>[4x]MSPEKQPLPAALVGSHVRAAAGTPADLATDRKFWTGLSRAVQERIADDWERTREAYGAARQQHYFSAEFLMGRALLNNLTNLGLVDEAAAATRELGHELTDILEIENDAALGNGGLGRLAACFLDSAVTQDYPVTGYGLLYRFGLFRQSFNEGFQVEKPDPWREEEYPFTIRRASDQLVVCFDDMKTRAIPYDMPITGYGTHNVGTLRLWKAEPWEEFDYDAFNAQRFTDAIIERERVSDICRVLYPNDTTYEGKKLRVRQQYFFTSASLQAMIQDHLAHH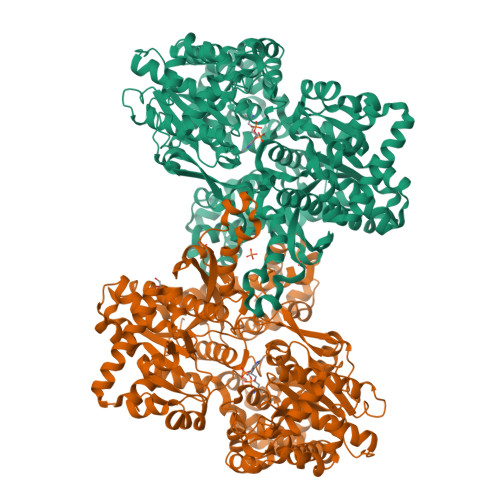KDLSNFAEFHSVQLNDTHPVLAIPELMRLLMDEHDMGWEESWAIVSKTFAYTNHTVLTEALEQWDEQIFQQLFWRVWEIIAEIDRRFRLERAADGLDEETINRMAPIQHGTVHMAWIACYAAYSINGVAALHTEIIKAETLADWYALWPEKFNNKTNGVTPRRWLRMINPGLSDLLTRLSGSDDWVTDLDELKKLRSYADDKSVLEELRAIKAANKQDFAEWILERQGIEIDPESIFDVQIKRLHEYKRQLMNALYVLDLYFRIKEDGLTDIPARTVIFGAKAAPGYVRAKAIIKLINSIADLVNNDPEVSPLLKVVFVENYNVSPAEHILPASDVSEQISTAGKEASGTSNMKFMMNGALTLGTMDGANVEIVDSVGEENAYIFGARVEELPALRESYKPYELYETVPGLKRALDALDNGTLNDNNSGLFYDLKHSLIHGYGKDASDTYYVLGDFADYRETRDRMAADYASDPLGWARMAWINICESGRFSSDRTIRDYATEIWKLEPTPAVKK>[4x]NEIVVYSARADELLKPIAEAYQQKTGTKVTVVSDKAGPLMERLKAEGKNTQADVLITVDGGNLWQATQAGVLRPINSSVLKSNIPSHLRDPKNHWFGLSVRARTIFYNPNKVNPSE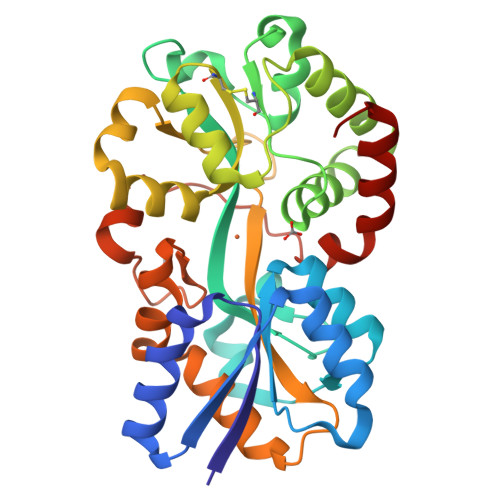LSTYADLADPKWKGRLCLRTSNNVYNQSLVATMIANHGQATTDRVVKGWVANLAAAPFANDTALLEAIDAGRCDVGIANTYYYGRLLNSKPQVANNVKVFFANQAGKGTHVNVSGAGVVKHSDNPAEAQKFIEWLSSNEAQRLYADRNFEYPANIQVTPTPAVARWGRFKQDFINVSVAGQNQQKAIMTMKRAGYK> MHHHHHHHHPDLGTGSENLYFQGAMADQVQDMYYLSPMQEGMLFHAILNPGQSFYLEQITMKVKGSLNIKCLEESMNVIMDRYDVFRTVFIHEKVKRPVQVVLKKRQFQIEEIDLTHLTGSEQTAKINEYKEQDKIRGFDLTRDIPMRAAIFKKAEESFEWVWSYHHIILDGWCFGIVVQDLFKVYNALREQKPYSLPPVKPYKDYIKWLEKQDKQASLRYWREYLEDFEGQTTFAEQRKKQKDGYEP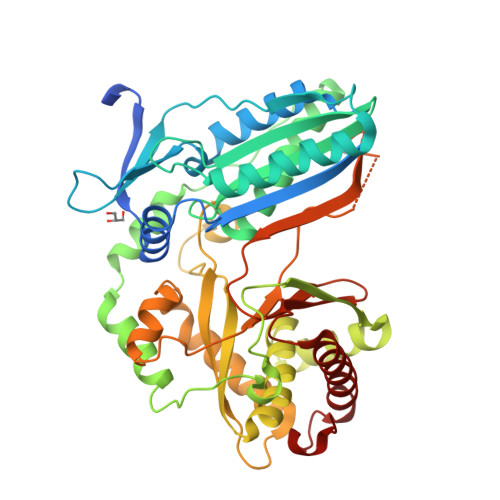KELLFSLPEAETKAFTELAKSQHTTLSTALQAVWSVLISRYQQSGDLAFGTVVSGRPAEIKGVEHMVGLFINVVPRRVKLSEGITFNDLLKQLQEQSLQSEPHQYVPLYDIQSQADQPKLIDHIIVFENYPLQDAKNEESSENGFDMVDVHVFEKSNYDLNLMASPGDEMLIKLAYNENVFDEAFILRLKSQLLTAIQQLIQNPDQPVSTINI> PGECSVNVIPKKNLDKAKFFSGTWYVTHYLDMDPQATEKFCFSFAPRESGGTVKEALYHFNVDSKVSFYNTGTGPLESNGAKYTAKFNTVDKKGKEIKPADEKYSYTVTVIEAAKQSALIHICLQEDGKDIGDLYSVLNRNKNALPNKKIKKALNKVSLVLTKFVVTKDLDCKYDDKFLSSWQK

Nitrophorins (NPs) comprise a unique class of ferrihemeproteins originating from the blood-feeding insect Rhodnius prolixus. They participate in the storage, transport, and delivery of nitric oxide (NO) from the insect to the bite site, where NO acts as a vasodilator and as an anticoagulant to facilitate the feeding process. The heme cofactor is located inside the central cavity of the lipocalin fold, which consists of an eight-stranded antiparallel β-barrel. Coordinated to the proximal His60, the heme iron is stable in the ferric form, whose NO affinity is low enough to make the release mechanism physiologically relevant.

The X-ray structure of NP7(E27V) was solved in order to examine the impact of the Glu27 mutation on the structure of the heme cavity. Data collection and refinement statistics of two X-ray structures solved for NP7(E27V) at pH 6.8, the aquo form and the complex with heme-bound imidazole (IMH), are provided in Supporting Information Table S1. The overall fold of NP7(E27V) closely resembles the 3D skeleton of wt NP7, as noted in the Root Mean Square Deviation (RMSD) values for the protein backbone (upon exclusion of the first three and last four residues) close to 0.2 Å for the two NP7(E27V) structures relative to the wt NP7. The AB and GH loops in NP7(E27V) closely fit the arrangement found in wt NP7 solved at both pH 5.8 and 7.818. However, this can be explained by the reduced conformational flexibility imposed by the head-to-tail arrangement of proteins in the crystal lattice, which involves numerous salt bridges between the clustering of Lys residues at the rear surface of the protein, and the negative charges located at the heme mouth. In contrast, NMR studies showed that NP7(E27V) mainly contains B-heme, although a significant fraction of A-heme was also found (ratio A:B of 1:3 at pH 5.5), thus revealing some degree of heme rotational disorder. Note that breakage of the Asp32-Ile132 HB was found even at the acidic conditions used in crystallization (pH 5.5), as was also found for the X-ray structure of wt NP79, suggesting that this structural feature likely reflects the disturbing effect caused by the head-to-tail electrostatic interactions in the crystal. The close resemblance between the X-ray structures of wt NP7 and NP7(E27V) may be misleading for interpreting the functional behavior of NP7 in solution, as key structural details, such as the heme orientation, the spatial layout of the AB loop, and the absence of a HB between Asp32 and Ile132 may be affected by the packing. However, the increase in the apparent rate of the bimolecular phase observed for wt NP7 as the pH is lowered to 5.5 is smaller for NP7(E27V) and becomes negligible for NP7(E27Q), indicating that annihilation of the negative charge of Glu27 upon mutation reduces the pH sensitivity of the ligand rebinding process.>[2x]SNAHMAPSAKDSEPATSCAAKKDSLNNYLWDLQYDKTNILARHGETIENKFSSDSFNKNGEFVVVEHQKKNIT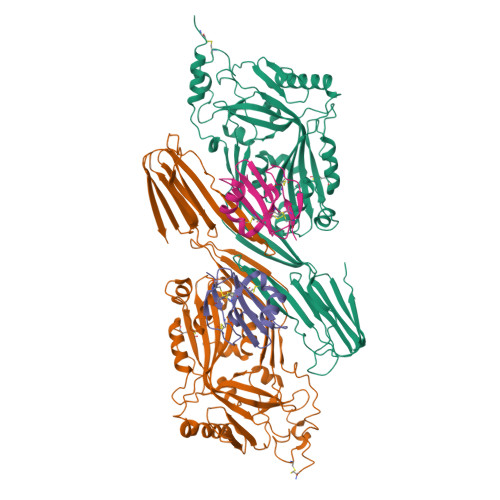NTTSNLSVTSANDDRVYPGALFRADKNLMDNMPSLISANRAPITLSVDLPGFHGGESAVTVQRPTKSSVTSAVNGLVSKWNAQYGASHHVAARMQYDSASAQSMNQLKAKFGADFAKIGVPLKIDFDAVHKGEKQTQIVNFKQTYYTVSVDAPDSPADFFAPCTTPDSLKNRGVDNKRPPVYVSNVAYGRSMYVKFDTTSKSTDFQAAVEAAIKGVEIKPNTEFHRILQNTSVCAVILGGSANGAAKVCTGNIDTLKALIQEGANLSTSSPAVPIAYTTSFVKDNEVATLQSNSDYIETKVSSYRNGYLTLDHRGAYVARYYIYWDEYGTEIDGTPYVRSRAWEGNGKYRTAHFNTTIQFKGNVRNLRIKLVEKTGLVWEPWRTVYDRSDLPLVRQRTISNWGTTLWPRVAETVKND;>MLQCYNCPNPTADCKTAVNCSSDFDACLITKAGLQVYNKCWKFEHCNFNDVTTRLRENELTYYCCKKDLCNFNEQLEN[2x]>[2x]DYLQQKRFLATSQGTTYVYDIPDMFRQMVERRWRECIEEGSVDGPQPDNVMTLVELVVEPDGERRVVEVTRLPGQNNVGMVAWRLTLYTPECPDGRDIVLIANDLTYYMGSFGPQEDWVYFKASQYARELKIPRIYISVNSGARIGVAEEVKSDFNVAWLDAERPERGFKYLYLTPEVYSKLGALGSVKTELIEDEGESRYRITDIIGKEDGLGVECLRDAGLIAGETAQAYEDIVTISIVTCRAIGIGSYIVRLGHRVIQVESSYIILTGYAALNKVLGRAVYASNNQLGGVQVMHHNGVSHAVAPSDLEAVRTALRWLAFVPKDKLSTVPILRVSDPVDRPVEWKPPRAAHDPRLMLAGDAAR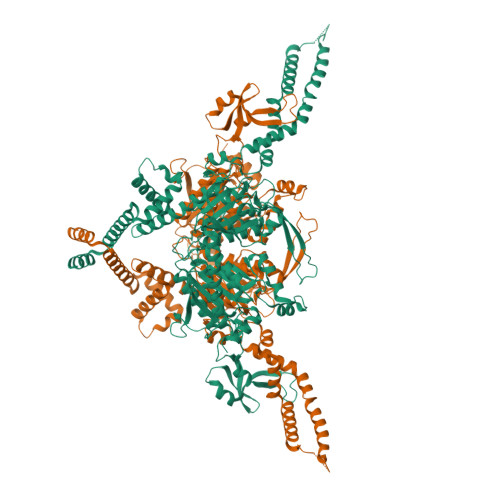AGFFDVGSFDEIMQPWAQTVITGRARLGGIPVGVIAVETRTVELTQPADPANLDSEAKTLQQAGQVWFPDSAYKTAQAINDFSRENLPIMIFANWRGFSGGQKDMYEQILKFGAEIVRALRGATAPVLVYIPPGAELRGGAWAVVDPSVNSLRMEMYADPEARGGVLEAEGIVEVKFKQRDILKTMHRLDPELLRTGARISELKEQIKEISKGLDRRGSVDESLIRTDAGRAAETRVRELETELLAAEKTAKAREKELSPIYHEIAVQFAELHDTAERMLEKGCIFEIIPWRDSRRLFYWRLKRLLRQNEQERRVQAAVKPADNMQQGPAAATLRRWFTEDRGETQSHQWEHDNEAVCKWLEAQAGDDNSVLERNLRAIHQDALMQAVNNLVLELTPSQRSEFIRKLSALEMEQ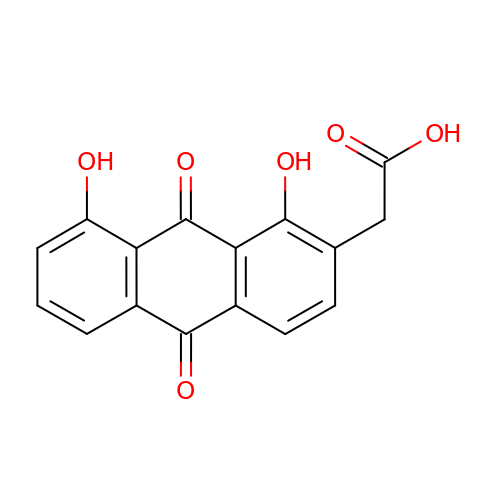(1,8-DIHYDROXY-9,10-DIOXO-9,10-DIHYDRO-ANTHRACEN-2-YL)-ACETIC ACID | C16 H10 O6 | IKFRFGXQHSBCQM-UHFFFAOYSA-N Pleckstrin is an intriguing platelet protein that appears to be involved in reorganization of the cytoskeleton, as well as attenuating various signaling pathways following platelet activation. On cloning pleckstrin, two internal repeats consisting of approximately 100 amino acids including 30 identical residues were identified at the N- and C-termini of the protein. The domain structure consists of a seven-stranded anti-parallel β-sandwich that is closed at one end by a C-terminal alpha helix and remains open at the other end, where several variable loop regions are located. Previous studies have shown that phosphatidylinositol 3,4-bisphosphate [PtdIns(3,4)P2] binds to C-PH much more firmly than other phosphoinositides and that IP6 is a potent inhibitor of pleckstrin-phosphoinositide interactions.

To investigate further the nature of the myo-inositol polyphosphate interaction with C-PH, crystals were prepared using recombinant C-PH and IP6, which permitted the determination of a high-resolution crystal structure. To our surprise, we found that the complex formed contained D-myo-inositol 1,2,3,5,6-pentakisphosphate [Ins(1,2,3,5,6)P5], rather than IP6. The resulting crystals were of exceptional quality and diffracted to 1.35 Å. The final model was well ordered with the exception of an approximately eight-residue loop region between the fifth and sixth beta strands, corresponding to residues 303–310. Ins(1,2,3,5,6)P5 was bound to C-PH in the β1–β2 loop region (residues 253–264 and 277), making numerous interactions through all but one of its phosphate groups. The only phosphate group that does not interact with any residues of C-PH is that in the 1-position of myo-inositol. The 2-phosphate is the only phosphate that adopts an axial position. This configuration is strongly stabilized through interactions with the side chains of R264 and K253. The 5-phosphate of Ins(1,2,3,5,6)P5 interacts with main chain atoms of H256, R257 and N260 (water-mediated), as well as the side chain of R257. Regardless of its source, Ins(1,2,3,5,6)P5 binds specifically in the phosphoinositide binding cleft of C-PH making numerous interactions with residues known to be involved in binding PtdIns(3,4)P2.

> GSFTGVIIKQGCLLKQGHRRKNWKVRKFILREDPAYLHYYDPAGAEDPLGAIHLRGCVVTSVESNSNGRKSEEENLFEIITADEVHYFLQAATPKERTEWIKAIQMASR3-nitrophenol | C6 H5 N O3 | 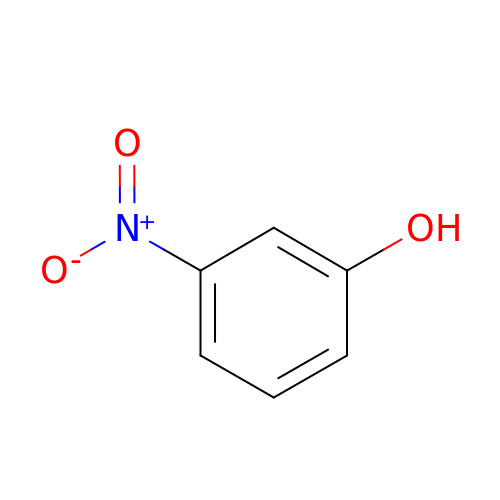RTZZCYNQPHTPPL-UHFFFAOYSA-N> MHHHHHHMVDEILKLKKEKGYIILAHN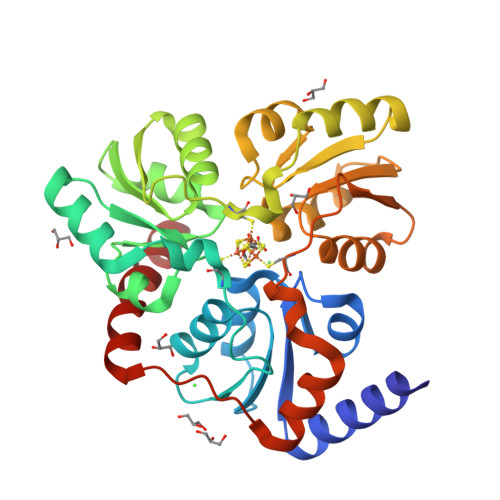YQIPELQDIADFVGDSLQLARKAMELSEKKILFLGVDFMAELVKILNPDKKVIVPDRSATCPMANRLTPEIIREYREKFPDAPVVLYVNSTSECKTLADVICTAANAVEVVKKLDSSVVIFGPDRNLGEYVAEKTGKKVITIPENGHCPVHQFNAESIDAVRKKYPDAKVIVHPECPKPVRDKADYVGSTGQMEKIPERDPSRIFVIGTEIGMIHKLKKKFPDREFVPLEMAVCVNMKKNTLENTLHALQTESFEVILPKEVIEKAKKPILRMFELMG> GSSNE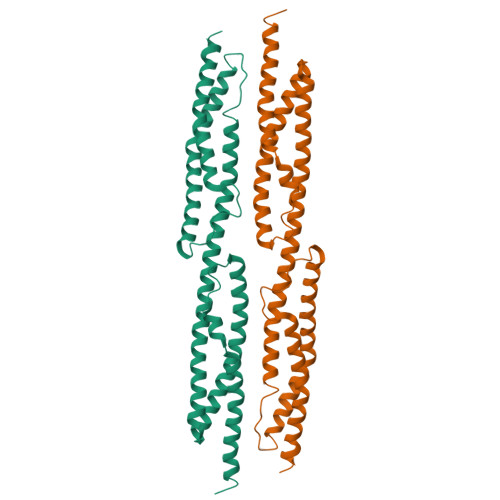IRRLERLEHLAEKFRQKASTHETWAYGKEQILLQKDYESASLTEVRALLRKHEAFESDLAAHQDRVEQIAAIAQELNELDYHDAVNVNDRCQKICDQWDRLGTLTQKRREALERMEKLLETIDQLHLEFAKRAAPFNNWMEGAMEDLQDMFIVHSIEEIQSLITAHEQFKATLPEADGERQSIMAIQNEVEKVIQSYNIRISSSNPYSTVTMDELRTKWDKVKQLVPIRDQSLQEELARQHANER> MGQIVTFFQEVPHVIEEVMNIVLIALSVLAVLKGLYNFATCGLVGL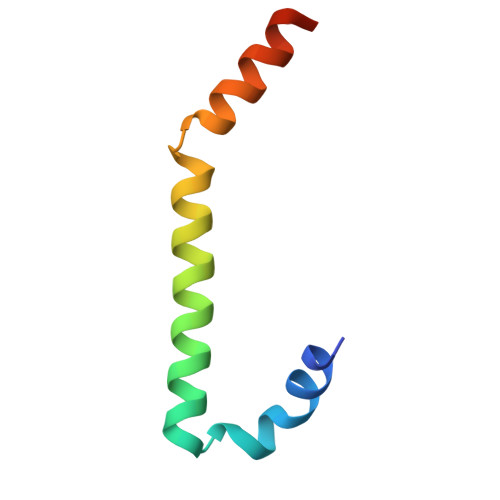VTFLLLCGRSCT> AAER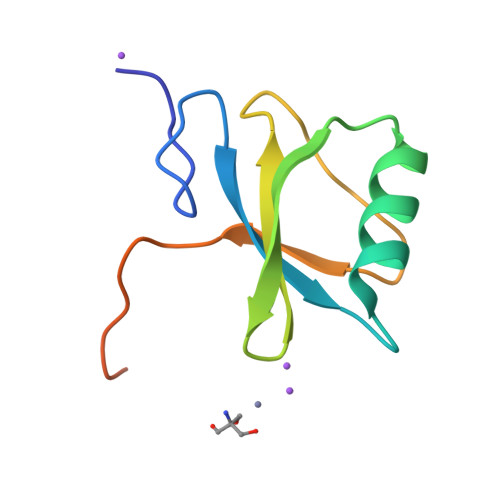SLLTGEEGWRTYKATGPRLSLPRLVALLKGQGLEVGKVAEAEGGFYVDLRPEARPEVAGLRLEPARRVEGLLEIPSRTRRPARA>[2x]MPV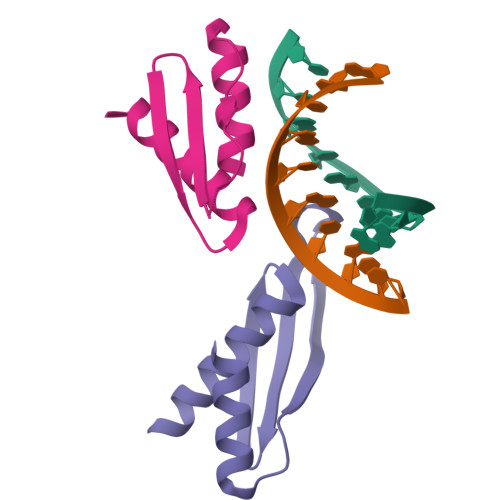GSLQELAVQKGWRLPEYTVAQESGPPHKREFTITCRVETFVETGSGTSKQVAKRVAAEKLLTKFKT>SAPVRLPFSGFRLQKVLRESARDKIIFLHGKVNEASGDGDGEDAVVILEKTPFQVEQVAQLLTGSPELQLQFSNDIYSTYHLFPPRQLNDVKTTVVYPATEKHLQKYLRQDLRLIRETGDDYRNITLPHLESQSLSIQWVYNILDKKAEADRIVFENPDPSDGFVLIPDLKWNQQQLDDLYLIAICHRRGIRSLRDLTPEHLPLLRNILHQGQEAILQ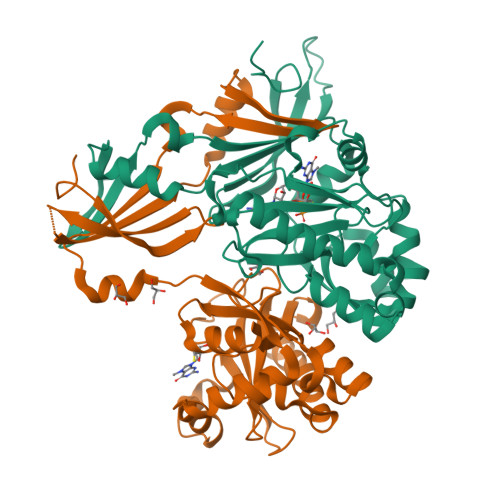RYRMKGDHLRVYLHYLPSYYHLHVHFTALGFEAPGSGVERAHLLAEVIENLECDPRHYQQRTLTFALRADDPLLKLLQEAQQS[2x]> GHMSHLADVSPPTACRVCGGGVQEFLDLGRQPLSDRFRKPDELDDEFTYRLAVGRCDSCEMVQLTEEVPRDLMFHEVYPYHS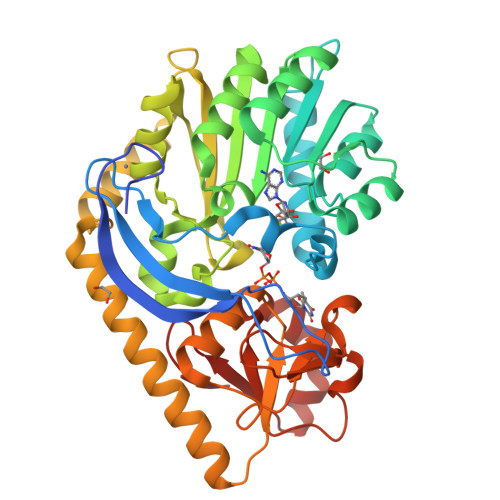SGSSVMREHFAMLARDFLATELTGPDPFIVEIGCNDGIMLRTIQEAGVRHLGFEPSSGVAAKAREKGIRVRTDFFEKATADDVRRTEGPANVIYAANTLCNIPYVQSVLEGVDALLAPDGVFVFEDPYLGDIVAKTSFDQIYDEHFFLFSATSVQGMAQRCGFELVDVQRLPVHGGEVRYTLARQGSRTPSAAVAQLLAAEREQELSDMATLRAFAGNVVKIRDELTALLHRLRAEGRSVVGYGATAKSATVTNFCGIGPDLVHSVYDTTPDKQNRLTPGAHIPVRPASAFSDPYPDYALLFAWNHAEEIMAKEQEFHQAGGRWILYVPEVHIR>[2x]MQWSGARALEALLTVAGELRGPPLQLDTGQLLKIAKRGGVTAVEAVHAWRNALTGAPLNLTPEQVVAIASHDGGKQALETVQRLLPVLCQAHGLTPQQVVAIASHDGGKQALETVQRLLPVLCQAHGLTPEQVVAIASHDGGKQALETVQALLPVL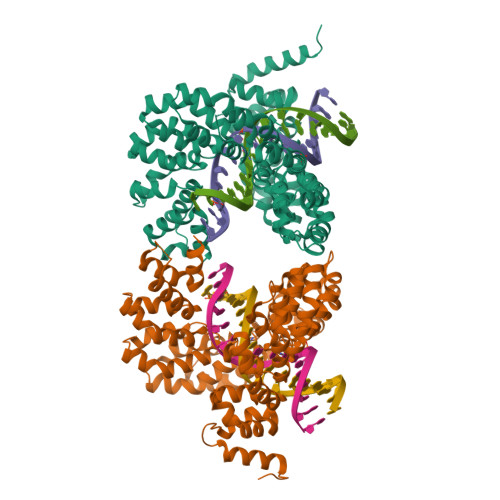CQAHGLTPEQVVAIASNGGGKQALETVQRLLPVLCQAHGLTPQQVVAIASNGGGKQALETVQRLLPVLCQAHGLTPQQVVAIASNGGGKQALETVQRLLPVLCQAHGLTPQQVVAIASNSGGKQALETVQRLLPVLCQAHGLTPQQVVAIASNGGGKQALETVQRLLPVLCQAHGLTPQQVVAIASHDGGKQALETVQRLLPVLCQAHGLTPEQVVAIASNGGGKQALETVQRLLPVLCQAHGLTPEQVVAIASHDGGKQALETVQRLLPVLCQAHGLTPQQVVAIASNGGGRPALESIVAQLSRPDPALAALTNDHLVALACLGGRPALDAVKKLEHHHHHH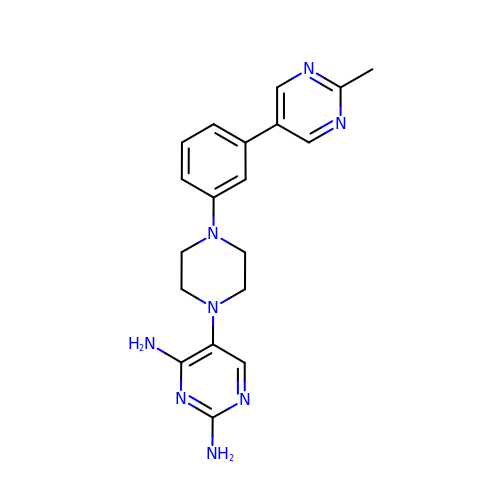5-{4-[3-(2-methylpyrimidin-5-yl)phenyl]piperazin-1-yl}pyrimidine-2,4-diamine | C19 H22 N8 | NLZHOJOCWCLWFT-UHFFFAOYSA-N> MTISTPVIIDSLIRHAQRTPEQTALLCGDQHWNYRQLVTRAHVMASALRQAGLSGQAILLNLPKSLDAVAAIYAT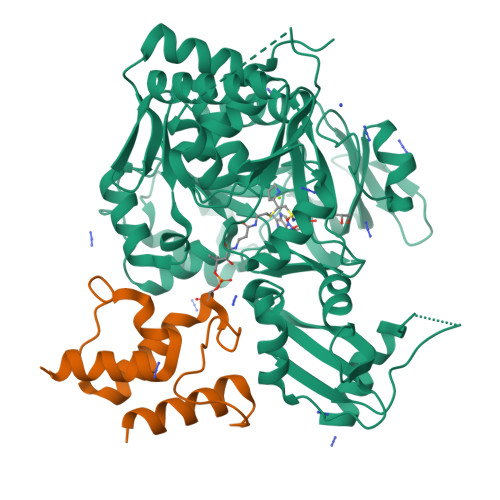WLSGNHYIPIDYSQPSSRIERIIAAAAPALIIDTAWLATLDSQPSFDAEQPVGRMVYHNPIAAILYTSGSTGTPKGVQISHEMLGFFIQWAVRDTQLTARDVLSNHASFAFDLSTFDLFASAYVGAATWIIRESEQKDCAALAQGLQRHAVSVWYSVPSILAMLEKSTLLNPTLGQSLRQVIFAGEPYPVTALKRLLPCLPQPCRVSNWYGPTETNVCVAYAIDRARLAMLKQVPIGLPLEGLTAQLEDENGDRHPLTAQLRLSGELLISGPCVTPGYSNVVVPRQAALHPHQCHATGDWVEMTPEGLVFRGRIDDMVKINGYRVELGEIESVLHQHPAIDRAALCVELGDLRQTLIMVISLQTGAVPPGLLELKQFLQQKLPSYMIPNKLVITESLPVNANGKVDRKQLAGVVAVLEHHHHHH;> MLESKLINHIATQFLDGEKDGLDSQTPLFELNIVDSAAIFDLVDFLRQESKVSIGMQEIHPANFATVQSMVALVQRLKAHPEQGGAAWEHHHHHH> MSLTREAYHRLTPLPHPGGRLFIKPGARGYRDPVHDLLQKTVEPFGERALDLNPGVGWGSLPLEGRMAVERLETSRAAFRCLTASGLQARLALPWEAAAGAYDLVVLALPAGRGTAYVQASLVAAARALRMGGRLYLAGDK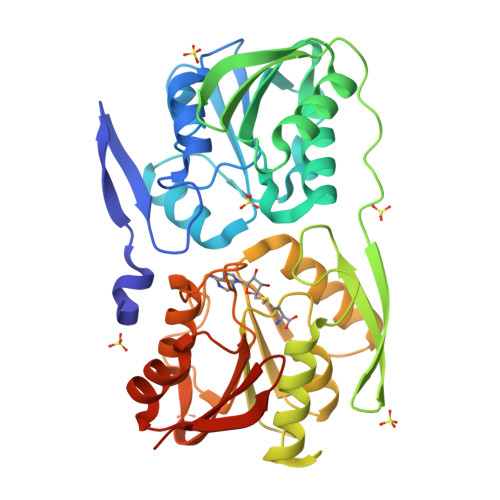NKGFERYFKEARALLGYGVVVRREGPYRVALLEKEKEAPPLPSLWRAFSARILGAEYTFHHLPGVFSAGKVDPASLLLLEALQERLGPEGVRGRQVLDLGAGYGALTLPLARMGAEVVGVEDDLASVLSLQKGLEANALKAQALHSDVDEALTEEARFDIIVTNPPFHVGGAVILDVAQAFVNVAAARLRPGGVFFLVSNPFLKYEPLLEEKFGAFQTLKVAEYKVLFAEKRGRHHHHHH1-[(2~{S})-2-(4-methoxyphenyl)pyrrolidin-1-yl]propan-1-one 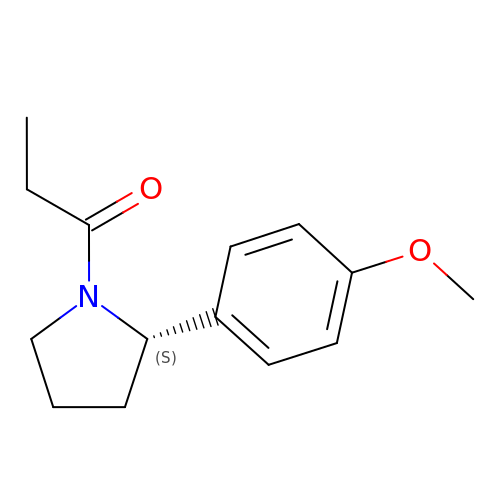| C14 H19 N O2 | WEJKDJNGWBEPQM-ZDUSSCGKSA-N> FQGAMSSSIDISKINSWNKEFQSDLTHQLATTVLKNYNADDALLNKTRLQKQDNRVFNTVVSTDSTPVTNQKSSGRCWLFAATNQLRLNVLSELNLKEFELSQAYLFFYDKLEKANYFLDQIVSSADQDIDSRLVQYLLAAPTEDGGQYSMFLNLVKKYGLIPKDLYGDLPYSTTASRKWNSLLTTKLREFAETLRTALKERSADDSIIVTLREQMQREIFRLMSLFMDIPPVQPNEQFTWEYVDKDKKIHTIKSTPLEFASKYAKLDPSTPVSLINDPRHPYGKLIKIDRLGNVL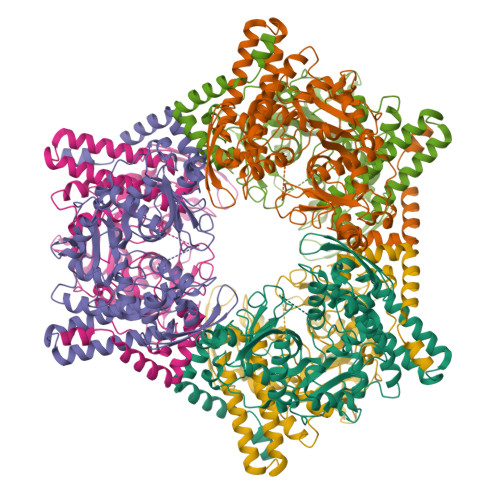GGDAVIYLNVDNETLSKLVVKRLQNNKAVFFGSHTPKFMDKKTGVMDIELWNYPAIGYNLPQQKASRIRYHESLMTHAMLITGCHVDETSKLPLRYRVEVSWGKDSGKDGLYVMTQKYFEEYCFQIVVDINELPKELASKFTSGKEEPIVLPIWDPMGALA4-(2-amino-6-{bis[(pyridin-2-yl)methyl]amino}pyrimidin-4-yl)phenol | C22 H20 N6 O | 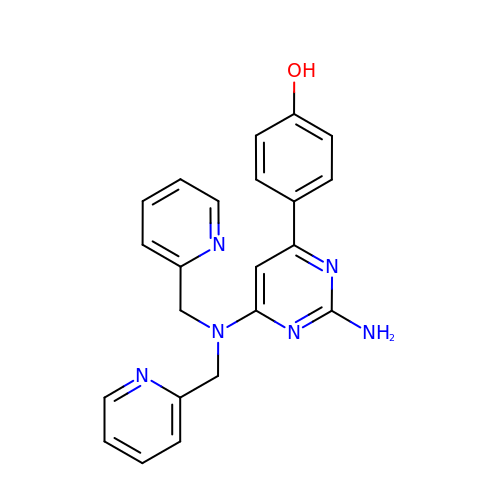LXSAXBJSZAHFFN-UHFFFAOYSA-N> IAPLVGYAIGAAAISAVGGIGVGWTLREFEVVGSDDPAEGLTPDVLRNQLSDSVVKRKSNNQSTMVDNQNILDGVEHTAYTEAKIAAIEELNAGSSESAVLSAANSAIDSYETTVRTNFYKSWNETVRELEAMTQTVIAHADVGLSYITDFGDPRFGNLASGTSPNTLKDTTVSMPDGTNFTLLTFRHNTGWDSGNAAYSVVEYNPKEVVTSTNSNTYNTVDGTQYMKFSEWNAVETEMDTVFQNVRNGISTWVTNVYGDVQS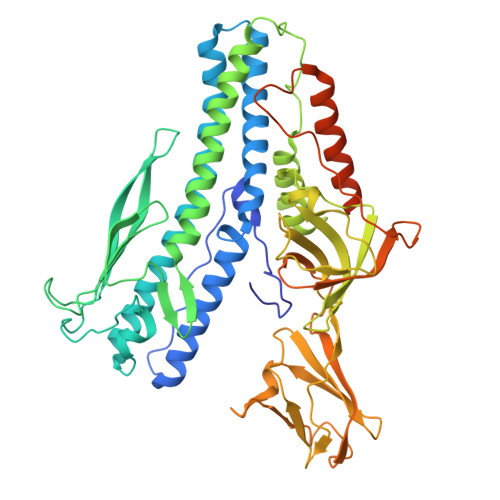GAIEISDLVTPRERATMMAQEEGMSQAIADLIALNVPVDAEREATITIQDTGATLPGTFALTDSSDGPLSAGQTYDPSTFSGDVYFTADMSLVEGPWDAINSGVDGGTITITSEPYEGTAIEVTTVESETVSVPAADWTDNGDGTWSYDASGDLETTITNVDSARFVSTATETTYDTLQLKGAFTVDKLVNKQSGEEVSSTSFTSSEPQTDSNYITQDEWDQLEQQNKELIEKYEQSQSGGGLDLGGLDMFGVPGEMVAVGAAAVIGFLMLGNN>SLPEGKIMPNTVFVGGIDVRMDETEIRSFFARYGSVKEVKIITDRTGVSKGYGFVSFYNDVDV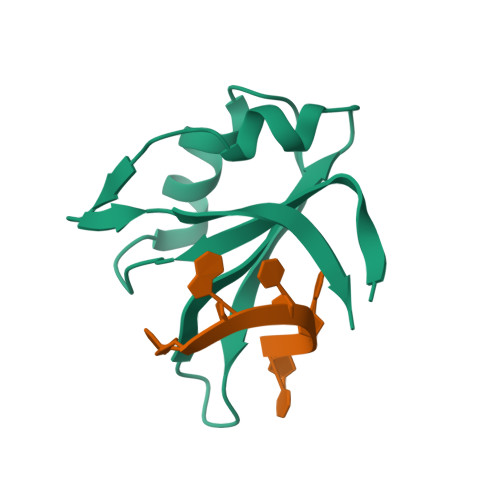QKIVESQINFHGKKLKLGPAIRKQ[2x]> SMADIGSTNDALDYYLKSKGFNGLFSQIELSFSASNLRDRDVLSKSDPMVVVYQKEKDATLSEVFRSEVVLNSLAPKWIKKFIVAYHFETVQTLVFRVYDVDTKFQNSREEMLKLDEQQFLGEATCALSEIITKSTRTSTLELKRKDGFAPQAQPHHGKLIIHAEESLASKISTEIVFRCSNLESKDLFSKSDPFLVVSKIVEHGTPIP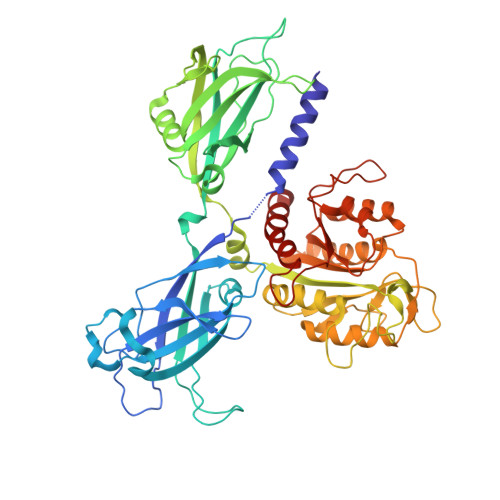VSKTEVRKNDLNPIWKPVFLSVQQVGSKDSPVIIECSDFNSNGKHSLIGKVQKSLSDLEKLHLAGQGINFSLPTGAGQNKVLKSQLFVDKFTETVHHTFLEYLASGFELNFMVAIDFTASNGNPRLPDSLHYIDPSGRLNAYQRAIMDVGEVLQFYDSDKRFPAWGFGARPIDAPVSHCFNLNGSSSYSEVDGIQGIMTSYTSALFNVSLAGPTLFGPVINAAAMIASASLAQGSRKYYVLLIITDGVITDLQETKDALVSASDLPLSILIVGVGGADFKEMEILDADKGERLESSSGRLASRDIVQFVALRDVQYGEISVVQALLAELPSQFLTYMRIRN Macrophage-expressed gene 1 (MPEG1, also termed Perforin-2) is one of the most ancient and highly conserved members of the membrane attack complex (MAC)/perforin-like (PF)/cholesterol-dependent cytolysin (MACPF/CDC) superfamily, with orthologous sequences identifiable throughout the metazoan. In contrast to other perforin-like proteins characterised to date, human MPEG1 is an integral type-1 transmembrane protein. The mature protein is comprised of three regions; an ectodomain located in the vesicular lumen, a transmembrane domain anchor that spans the vesicular membrane and, finally, a short cytosolic sequence. Each monomer of the 16-subunit ring possesses an N-terminal MACPF/CDC domain, a central multi-vesicular body of 12 kDa (MVB12)-associated β-prism (MABP) domain and a C-terminal region (termed the L-domain).

We therefore expressed the human MPEG1 ectodomain in order to investigate its function. Electron microscopy experiments revealed that the majority of recombinant material eluted as a stable multimeric complex. Accordingly, an integrative single particle cryo-EM approach was used to elucidate the structure of this assembly. Our initial efforts yielded a 3.5 Å structure of wild-type MPEG1. These data revealed that MPEG1 formed hexadecameric rings stacked together to form a double ring (or head-to-head assembly). Although this structure was incomplete, particularly in the C-terminal region, these data provided a platform for directed mutagenesis.

>[16x]KSGKPSGEMDEVGVQKCKNALKLPVLEVLPGGGWDNLRNVDMGRVMELTYSNCRTTEDGQYIIPDEIFTIPQKQSNLEMNSEILESWANYQSSTSYSINTELSLFSKVNGKFSTEFQRMKTLQVKDQAITTRVQVRNLVYTVKINPTLELSSGFRKELLDISDRLENNQTRMATYLAELLVLNYGTHVTTSVDAGAALIQEDHLRASFLQDSQSSRSAVTASAGLAFQNTVNFKFEENYTSQNVLTKSYLSNRTNSRVQSIGGVPFYPGITLQAWQQGITNHLVAIDRSGLPLHFFINPNMLPDLPGPLVKKVSKTVETAVKRYYTFNTYPGCTDLNSPNFNFQANTDDGSCEGKMTNFSFGGVYQECTQLSGNRDVLLCQKLEQKNPLTGDFSCPSGYSPVHLLSQIHEEGYNHLECHRKCTLLVFCKTVCEDVFQVAKAEFRAFWCVASSQVPENSGLLFGGLFSSKSINPMTNAQSCPAGYFPLRLFENLKVCVSQDYELGSRFAVPFGGFFSCTVGNPLVDPAISRDLGAPSLKKCPGGFSQHPALISDGCQVSYCVKSGLFTGGSLPPARLPPFTRPPLMSQAATNTVIVTNSENARSWIKDSQTHQWRLGEPIELRRAMNVIHGDGGGLSHHHHHH> ATCDDGRTTANAACCILFPILDDIQENLFDGAQCGEEVHESLRLTFHDAIGFSPTLGGGGADGSIIAFDTIETNFPANAGIDEIVSAQKPFVAKHNISAGDFIQFAGAVGVSNCPGGVRIPFFLGRPDAVAASPDHLVPEPFDSVDSILARMGDAGFSPVEVVYLLASHSIAAADKVDPSIPGTPFDSTPGVFDSQFFIETQLKGRLFPGTADNKGEAQSPLQGEIRLQSDHLLARDPQTACEWQSMVNNQPKIQNRFAATMSKMALLGQDKTKLIDCSDVIPT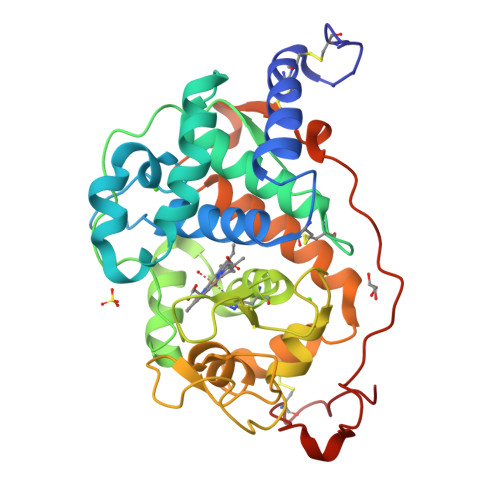PPALVGAAHLPAGFSLSDVEQACAATPFPALT>[2x]MKKYTCTVCVYIYNPEDGDPDNGVN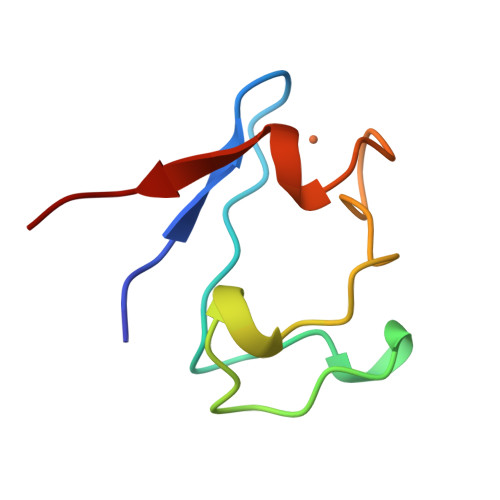PGTDFKDIPDDWVCPLCAVGKDQFEEVEE>[2x]MGSSHHHHHHSSGLVPRGSTSEVIEDEK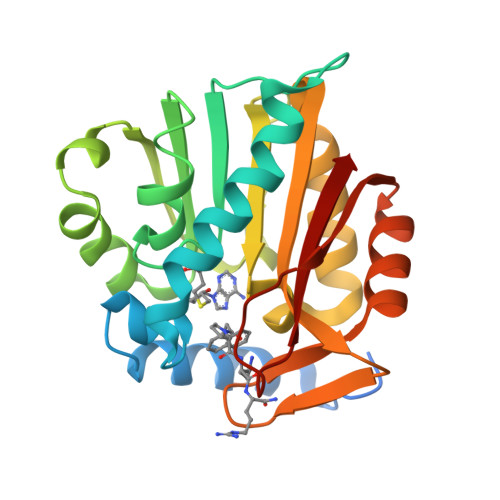QFYSKAKTYWKQIPPTVDGMLGGYGHISSIDINSSRKFLQRFLREGPNKTGTSCALDCGAGIGRITKRLLLPLFREVDMVDITEDFLVQAKTYLGEEGKRVRNYFCCGLQDFTPEPDSYDVIWIQWVIGHLTDQHLAEFLRRCKGSLRPNGIIVIKDNMAQEGVILDDVDSSVCRDLDVVRRIICSAGLSLLAEERQENLPDEIYHVYSFALR2-deoxy-2-{[(S)-hydroxy(methyl)phosphoryl]amino}-beta-D-glucopyranose | C7 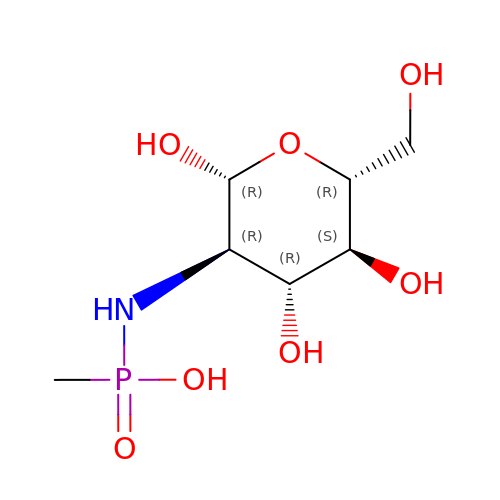H16 N O7 P | LKDVLOHRQALDHT-NYMZXIIRSA-N> XSLLEKLAEELRQLADELNKKF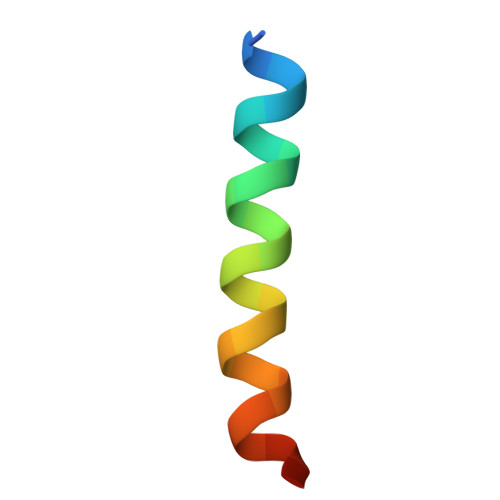EKX>[3x]PPGPPGPPGPRGDKGETGERG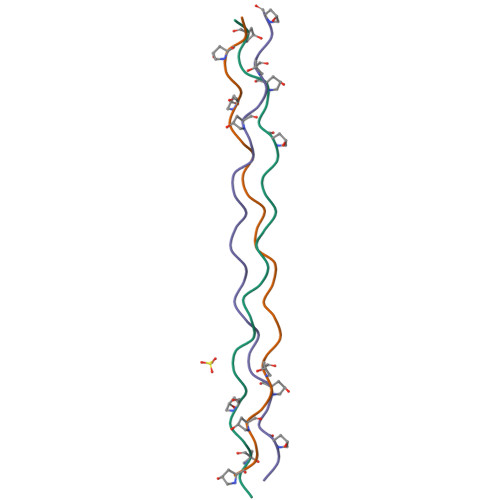PPGPPGPPG>MTSASNPPAFRLETSDGDEEGSAEVNKGKNEPPPMESPFQGEDRNFSPQIKVNLNYRKGLGPSQQDPNRFDRDRLFSVVSRGVPEELTGLLEYLRRTSKYLTDSAYTEGSTGKTCLMKAVLNLQDGVNACILPLLQIDRDSGNPQPLVNAQCTDEFYRGHSALHIAIEKRSLWCVKLLVENGANVHIRACGRFFQKHQGTCFYFGELPLSLAACTKQWDVVTYLLENPHQPASLEATDSLGNTVLHALVMIADNSPENSALVIHMYDSLLQMGARLCPTVQLEDICNHQGLTPLKLAAKEGKIEIFRHILQREFSGLYQPLSRKFTEWCYGPVRVSLYDLSSVDSWEKNSVLEIIAFHCKSPHRHRMVVLEPLNKLLQEKWDRLIPRFFFNFACYLVYMIIFTIVAYHQPSLEQPAIPSSKATFGDSMLLLGHILILLGGIYLLLGQLWYFWRRRLFIWISFMDSYFEILFLVQALLTVLSQVLRFVETEWYLPLLVSSLVLGWLNLLYYTRGFQHTGIYSVMITKVILRDLLRFLLVYLVFLFGFAVA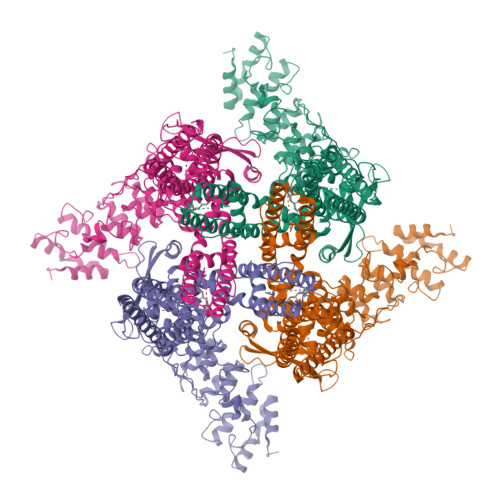LVSLSREARSPKAPEDSNTTVTEKPTLGQEEEPVPYGGILDASLELFKFTIGMGELAFQEQLRFRGVVLLLLLAYVLLTYVLLLNMLIALMSETVNSVATDSWSIWKLQKAISVLEMENGYWWCRRKRHRAGRLLKVGTKGDGIPDERWCFRVEEVNWAAWEKTLPTLSEDPSGAGITGYKKNPTSKPGKNSASEEDHLPLQVLQSH[4x]> MGSSHHHHHHSSGRENLYFQGHMRRGLVIVGHGSQLNHYREVMELHRKRIEESGAFDEVKIAFAARKRRPMPDEAIREMNCDIIYVVPLFISYGLHVTEDLPDLLGFPRGRGI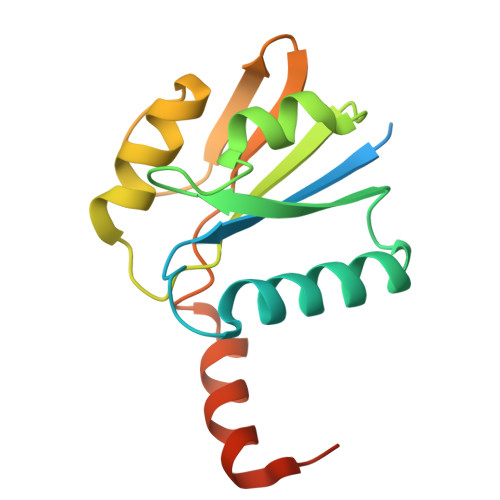KEGEFEGKKVVICEPIGEDYFVTYAILNSVFRIGRDGKGEEGS> GGUCAAGAUAGUAAGGGUCCACGGUGGAUGCCCUGGCGCUGGAGCCGAUGAAGGACGCGAUUACCUGCGAAAAGCCCCGACGAGCUGGAGAUACGCUUUGACUCGGGGAUGUCCGAAUGGGGAAACCCACCUCGUAAGAGGUAUCCGCAAGGAUGGGAACUCAGGGAACUGAAACAUCUCAGUACCUGAAGGAGAAGAAAGAGAAUUCGAUUCCGUUAGUAGCGGCGAGCGAACCCGGAUCAGCCCAAACCGAAACGCUUGCGUUUCGGGGUUGUAGGACCAGUUUUUAAGAUUCAACCCCUCAAGCCGAAGUGGCUGGAAAGCUACACCUCAGAAGGUGAGAGUCCUGUAGGCGAACGAGCGGUUGACUGUACUGGCACCUGAGUAGGUCGUUGUUCGUGAAACGAUGACUGAAUCCGCGCGGACCACCGCGCAAGGCUAAAUACUCCCAGUGACCGAUAGCGCAUAGUACCGUGAGGGAAAGGUGAAAAGAACCCCGGGAGGGGAGUGAAAGAGAACCUGAAACCGUGGACUUACAAGCAGUCAUGGCACCUUAUGCGUGUUAUGGCGUGCCUAUUGAAGCAUGAGCCGGCGACUUAGACCUGACGUGCGAGCUUAAGUUGAAAAACGGAGGCGGAGCGAAAGCGAGUCCGAAUAGGGCGGCAUUAGUACGUCGGGCUAGACUCGAAACCAGGUGAGCUAAGCAUGACCAGGUUGAAACCCCCGUGACAGGGGGCGGAGGACCGAACCGGUGCCUGCUGAAACAGUCUCGGAUGAGUUGUGUUUAGGAGUGAAAAGCUAACCGAACCUGGAGAUAGCUAGUUCUCCCCGAAAUGUAUUGAGGUACAGCCUCGGAUGUUGACCAUGUCCUGUAGAGCACUCACAAGGCUAGGGGGCCUACCAGCUUACCAAACCUUAUGAAACUCCGAAGGGGCACGCGUUUAGUCCGGGAGUGAGGCUGCGAGAGCUAACUUCCGUAGCCGAGAGGGAAACAACCCAGACCAUCAGCUAAGGUCCCUAAAUGAUCGCUCAGUGGUUAAGGAUGUGUCGUCGCAUAGACAGCCAGGAGGUUGGCUUAGAAGCAGCCACCCUUCAAAGAGUGCGUAAUAGCUCACUGGUCGAGUGACGAUGCGCCGAAAAUGAUCGGGGCUCAAGUGAUCUACCGAAGCUAUGGAUUCAACUCGCGAAGCGAGUUGUCUGGUAGGGGAGCGUUCAGUCCGCGGAGAAGCCAUACCGGAAGGAGUGGUGGAGCC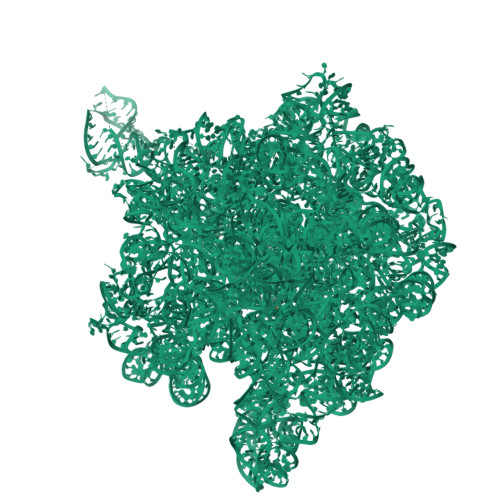GACUGAAGUGCGGAUGCCGGCAUGAGUAACGAUAAAAGAAGUGAGAAUCUUCUUCGCCGUAAGGACAAGGGUUCCUGGGGAAGGGUCGUCCGCCCAGGGAAAGUCGGGACCUAAGGUGAGGCCGAACGGCGCAGCCGAUGGACAGCAGGUCAAGAUUCCUGCACCGAUCAUGUGGAGUGAUGGAGGGACGCAUUACGCUAUCCAAUGCCAAGCUAUGGCUAUGCUGGUUGGUACGCUCAAGGGCGAUCGGGUCAGAAAAUCUACCGGUCACAUGCCUCAGACGUAUCGGGAGCUUCCUCGGAAGCGAAGUUGGAAACGCGACGGUGCCAAGAAAAGCUUCUAAACGUUGAAACAUGAUUGCCCGUACCGCAAACCGACACAGGUGUCCGAGUGUCAAUGCACUAAGGCGCGCGAGAGAACCCUCGUUAAGGAACUUUGCAAUCUCACCCCGUAACUUCGGAAGAAGGGGUCCCCACGCUUCGCGUGGGGCGCAGUGAAUAGGCCCAGGCGACUGUUUACCAAAAUCACAGCACUCUGCCAACACGAACAGUGGACGUAUAGGGUGUGACGCCUGCCCGGUGCCGGAAGGUCAAGUGGAGCGGUGCAAGCUGCGAAAUGAAGCCCCGGUGAACGGCGGCCGUAACUAUAACGGUCCUAAGGUAGCGAAAUUCCUUGUCGGGUAAGUUCCGACCUGCACGAAAGGCGUAACGAUCUGGGCGCUGUCUCAACGAGGGACUCGGUGAAAUUGAAUUGGCUGUAAAGAUGCGGCCUACCCGUAGCAGGACGAAAAGACCCCGUGGAGCUUUACUAUAGUCUGGCAUUGGGAUUCGGGUUUCUCUGCGUAGGAUAGGUGGGAGCCUGCGAAACUGGCCUUUUGGGGUCGGUGGAGGCAACGGUGAAAUACCACCCUGAGAAACUUGGAUUUCUAACCUGAAAAAUCACUUUCGGGGACCGUGCUUGGCGGGUAGUUUGACUGGGGCGGUCGCCUCCCAAAAUGUAACGGAGGCGCCCAAAGGUCACCUCAAGACGGUUGGAAAUCGUCUGUAGAGCGCAAAGGUAGAAGGUGGCUUGACUGCGAGACUGACACGUCGAGCAGGGAGGAAACUCGGGCUUAGUGAACCGGUGGUACCGUGUGGAAGGGCCAUCGAUCAACGGAUAAAAGUUACCCCGGGGAUAACAGGCUGAUCUCCCCCGAGAGUCCAUAUCGGCGGGGAGGUUUGGCACCUCGAUGUCGGCUCGUCGCAUCCUGGGGCUGAAGAAGGUCCCAAGGGUUGGGCUGUUCGCCCAUUAAAGCGGCACGCGAGCUGGGUUCAGAACGUCGUGAGACAGUUCGGUCUCUAUCCGCUACGGGCGCAGGAGAAUUGAGGGGAGUUGCUCCUAGUACGAGAGGACCGGAGUGAACGGACCGCUGGUCUCCCUGCUGUCGUACCAACGGCACAUGCAGGGUAGCUAUGUCCGGAACGGAUAACCGCUGAAAGCAUCUAAGCGGGAAGCCAGCCCCAAGAUGAGUUCUCCCACUGUUUAUCAGGUAAGACUCCCGGAAGACCACCGGGUUAAGAGGCCAGGCGUGCACGCAUAGCAAUGUGUUCAGCGGACUGGUGCUCAUCAGUCGAGGUCUUGACCACUC;> ACCA6-NITROINDAZOLE | C7 H5 N3 O2 | 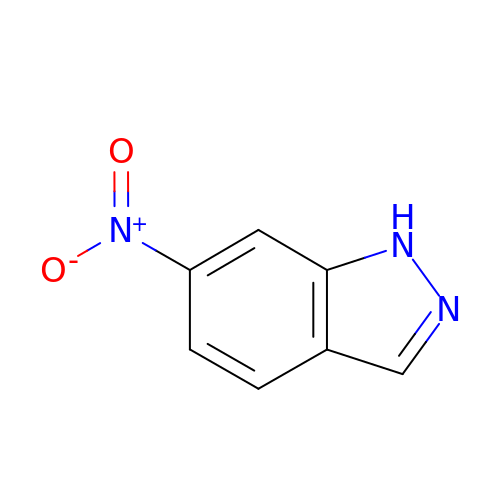ORZRMRUXSPNQQL-UHFFFAOYSA-N>SSSQKKAGGKAGKPT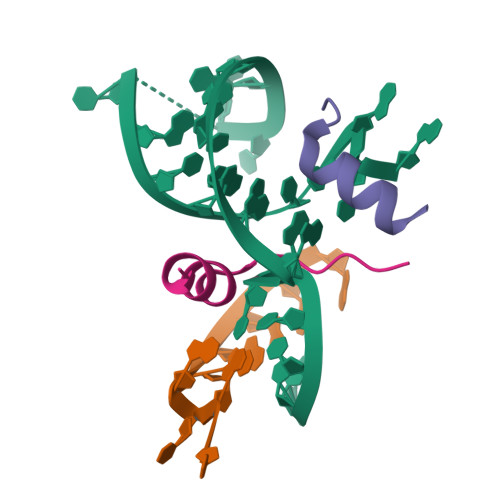KRSQNYAALRK[2x]> GAMAKPCDLP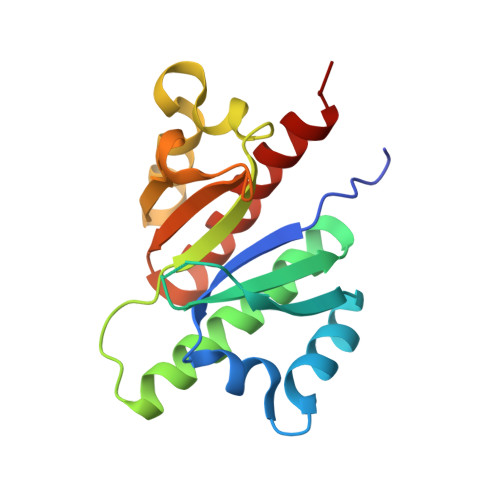LRLLVPTQFVGAIIGKEGATIRNITKQTQSKIDVHRKENAGAAEKSITILSTPEGTSAACKSILEIMHKEAQDIKFTEEIPLKILAHNNFVGRLIGDDGRNLKKIEQDTDTKITISPLQELTLYNPERTITVKGNVETCAKAEEEIMKKIRESYENDI> GALTESQAALVKSSWEEFNANIPKHTHRFFILVLEIAPAAKDLFSFLKGTSEVPQNNPELQAHAGKVFKLV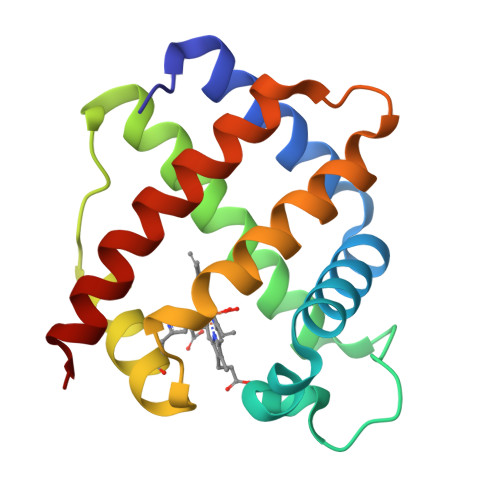YEAAIQLEVTGVVVTDATLKNLGSVHVSKGVADAHFPVVKEAILKTIKEVVGAKWSEELNSAWTIAYDELAIVIKKEMDDAA2-([1,1'-biphenyl]-4-yl)-3-methyl-1,7-naphthyridine-4-carboxylic 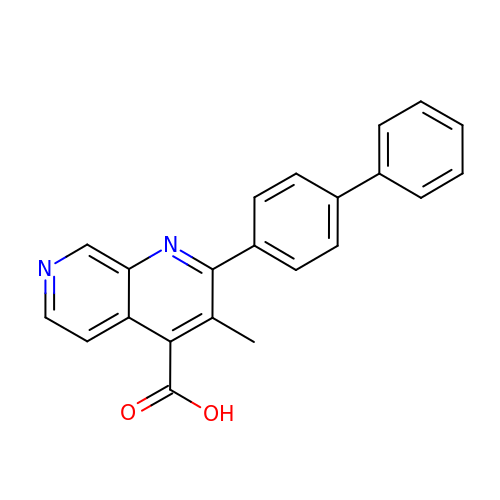acid | C22 H16 N2 O2 | QTJZVPVLAFKPGP-UHFFFAOYSA-N> MNITKPFPLPTGYFGIPLGLAALSLAWFHLENLFPAARMVSDVLGIVASAVWILFILMYAYKLRYYFEEVRAEYHSPVRFSFIALIPITTMLVGDILYRWNPLIAEVLIWIGTIGQLLFSTLRVSELWQGGVFEQKSTHPSFYLPAVA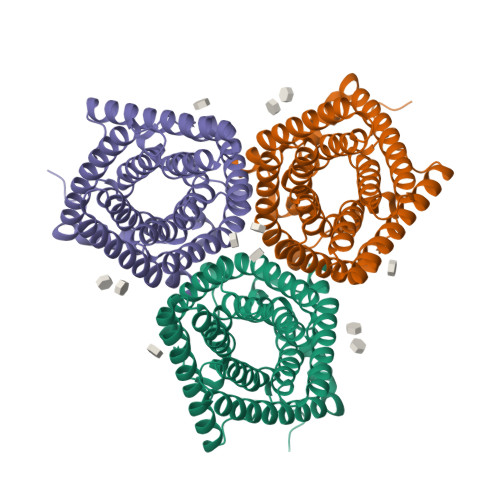ANFTSASSLALLGYHDLGYLFFGAGMIAWIIFEPVLLQHLRISSLEPQFRATMGIVLAPAFVCVSAYLSINHGEVDTLAKILWGYGFLQLFFLLRLFPWIVEKGLNIGLWAFSAGLASMANSATAFYHGNVLQGVSIFAFVFSNVMIGLLVLMTIYKLTKGQFFLK> MPGLSCRFYQHKFPEVEDVVMVNVRSIAEMGAYVSLLEYNNIEGMILLSELSRRRIRSINKLIRIGRNECVVVIRVDKEKGYIDLSKRRVSPEEAIKCEDKFTKSKTVYSILRHVAEVLEYTKDEQLESLFQRTAWVFDDKYKRPGYGAYDAFKHAVSDPSILDSLDLNEDEREVLINNINRRLTPQAVKI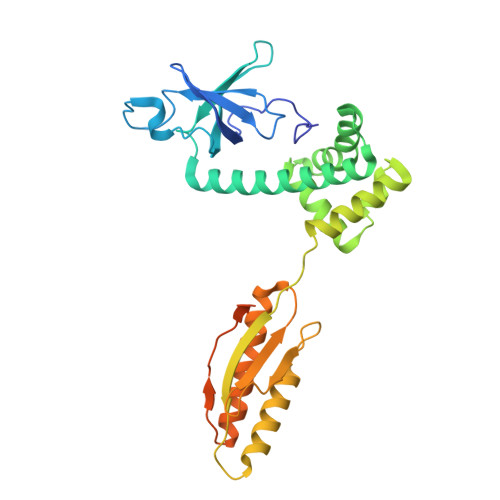RADIEVACYGYEGIDAVKEALRAGLNCSTENMPIKINLIAPPRYVMTTTTLERTEGLSVLSQAMAVIKEKIEEKRGVFNVQMEPKVVTDTDETELARQMERLERENAEVDGDDDAEEMEAKAED Endoglycosidase S (EndoS) secreted from Streptococcus pyogenes is a 108 kDa enzyme that specifically catalyzes the hydrolysis of the β-1,4 linkage between the first two N-acetylglucosamine residues of the complex-type N-linked glycan located on N297 of the Fc region of IgG antibodies. The presence of this N-linked glycan is critical for IgG function, contributing both to Fc γ receptor binding and activation of the complement pathway. EndoS belongs to family GH18, for which a substrate-assisted mechanism, with retention of the anomeric configuration, has been proposed. Altogether, our data provide critical insights into the structural determinants of complex-type N-linked glycan specificity of EndoS, a key event for S. pyogenes to evade the host immune system.

EndoSD233A/E235L crystallized in the P21 space group, with one molecule in the asymmetric unit and diffracted to a maximum resolution of 2.9 Å. The EndoS glycosidase domain adopts a (β/α)8-barrel topology with a long cavity that runs parallel to the protein surface in which one molecule of the G2 glycan product is unambiguously identified in the crystal structure. Two well-defined asymmetric grooves accommodate each of the complex-type N-linked glycan antennae: the Galβ1–4GlcNAcβ1–2Manα1–6 and Galβ1–4GlcNAcβ1–2Manα1–3 arms occupy grooves 1 and 2, respectively, both attached to the disaccharide Manβ1–4GlcNAc of the G2 product. The reducing end of the core Manβ1–4GlcNAc disaccharide is located at the end of the long cavity flanked by loops 4, 5, 6, and 7, and several residues from the β-barrel core. W153 is positioned in such a way as to engage the entire G2 trimannose core including the central Man (−2), the α(1–6)-linked Man (−3) and the α(1–3)-linked Man (−7). The terminal GlcNAc (−4 and −8) and Gal (−5 and −9) residues of each arm adopt two alternative conformations into the crystal structure. In one state, the GlcNAc (−4 and −8) and Gal (−5 and −9) residues protrude away from grooves 1 and 2, which may reflect the release of the G2 product from the active site; in the other state, these carbohydrates reside within their corresponding grooves, likely reflecting the binding mode of the G2 substrate. The structural comparison between the full-length EndoSD233A/E235L-G2 and the truncated unliganded version ΔN-3HB-EndoS suggests an important contribution of the N-3HB domain to stabilize the GH domain and generate a completely competent glycan binding site.

> MEEKTVQVQKGLPSIDSLHYLSENSKKEFKEELSKAGQESQKVKEILAKAQQADKQAQELAKMKIPEKIPMKPLHGPLYGGYFRTWHDKTSDPTEKDKVNSMGELPKEVDLAFIFHDWTKDYSLFWKELATKHVPKLNKQGTRVIRTIPWRFLAGGDNSGIAEDTSKYPNTPEGNKALAKAIVDEYVYKYNLDGLDVAVLHDSIPKVDKKEDTAGVERSIQVFEEIGKLIGPKGVDKSRLFIMDSTYMADKNPLIERGAPYINLLLVQVYGSQGEKGGWEPVSNRPEKTMEERWQGYSKYIRPEQYMIGFSFYEENAQEGNLWYDINSRKDEDKANGINTDITGTRAERYARWQPKTGGVKGGIFSYAIDRDGVAHQPKKYAKQKEFKDATDNIFHSDYSVSKALKTVMLKDKSYDLIDEKDFPDKALREAVMAQVGTRKGDLERFNGTLRLDNPAIQSLEGLNKFKKLAQLDLIGLSRITKLDRSVLPANMKPGKDTLETVLETYKKDNKEEPATIPPVSLKVSGLTGLKELDLSGFDRETLAGLDAATLTSLEKVDISGNKLDLAPGTENRQIFDTMLSTISNHVGSNEQTVKFDKQKPTGHYPDTYGKTSLRLPVANEKVDLQSQLLFGTVTNQGTLINSEADYKAYQNHKIAGRSFVDSNYHYNNFKVSYENYTVKVTDSTLGTTTDKTLATDKEETYKVDFFSPADKTKAVHTAKVIVGDEKTMMVNLAEGATVIGGSADPVNARKVFDGQLGSETDNISLGWDSKQSIIFKLKEDGLIKHWRFFNDSARNPETTNKPIQEASLQIFNIKDYNLDNLLENPNKFDDEKYWITVDTYSAQGERATAFSNTLNNITSKYWRVVFDTKGDRYSSPVVPELQILGYPLPNADTIMKTVTTAKELSQQKDKFSQKMLDELKIKEMALETSLNSKIFDVTAINANAGVLKDCIEKRQLLKKLGSGKILHNQNVNSWGPITVTPTTDGGETRFDGQIIVQMENDPVVAKAAANLAGKHAESSVVVQLDSDGNYRVVYGDPSKLDGKLRWQLVGHGRDHSETNNTRLSGYSADELAVKLAKFQQSFNQAENINNKPDHISIVGCSLVSDDKQKGFGHQFINAMDANGLRVDVSVRSSELAVDEAGRKHTKDANGDWVQKAENNKVSLSWDAQLEGGSGGSGNSGHHHHHHHHHH> SMKLDIKKTFSNRSDRVKGIDFHPTEPWVLTTLYSGRVEIWNYETQVEVRSIQVT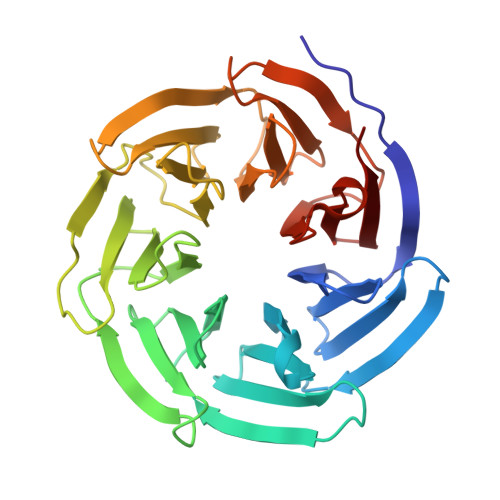ETPVRAGKFIARKNWIIVGSDDFRIRVFNYNTGEKVVDFEAHPDYIRSIAVHPTKPYVLSGSDDLTVKLWNWENNWALEQTFEGHEHFVMCVAFNPKDPSTFASGCLDRTVKVWSLGQSTPNFTLTTGQERGVNYVDYYPLPDKPYMITASDDLTIKIWDYQTKSCVATLEGHMSNVSFAVFHPTLPIIISGSEDGTLKIWNSSTYKVEKTLNVGLERSWCIATHPTGRKNYIASGFDNGFTVLSLG>MDMKEWEIFYNKIMEDFGFDKDKDVESAVILNNILENANTIPVDKLKDIIEGREVFIFGAGPSIKKHINILKELREINYKNPIIVADGACKAFLEENIIPDIIVSDLDGDLEALFECNRKGSIIVVHAHGDNIEKIKKYVPKLKN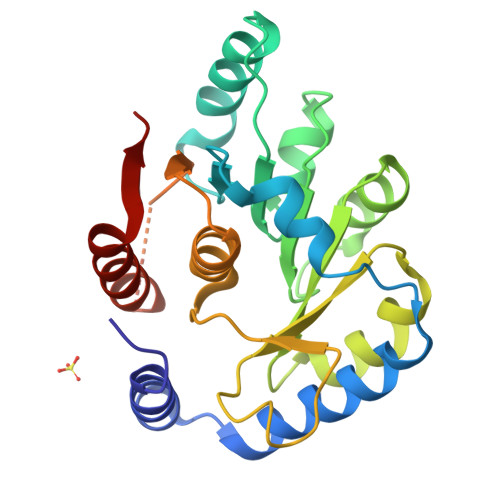VVGSCQIPNYKELNLRNVINFGGFTDGDRCCFLAYHFKAKKLILGGMDFGIYITKYSRPNIKEDIAIGDEIKIKKLEYAKTLINYLKDKIEIEFLK[4x]>[2x]MGSSHHHHHHSSGLVPRGSHDLSEGYVFGMGNPLLDIIVDADDFMYRKYNLKKDNIVLAEEKHMTIYDEIQKKKKLNYIAGGATLNTVKMIQWIIQKPFVCSYVG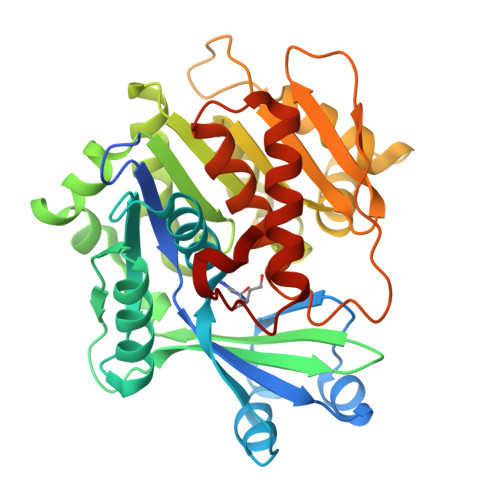CIGADIQGKYIKNDCSALDLVTEFQIAEEPLMTGKVAVLVSEKLRSMVTYLGAACDLSLAHIEQPHVWSLVEKAQVYYIAGFVINTCYEGMLKIAKHSLENEKLFCFNLSAPFLSQFNTKEVDEMISYSNIVFGNESEAEAYGEVHGLLEDTVHATARYIADLPFADGKKRKRLVIITRGKNPLLYTDSSDSEIHQFMVEQFKDDQIIDTNGAGDAFAAGFIADYIRGKPMITSLHAAVKAAAYIICRSGFSLGSRDSYSLKINK>[5x]ALAGTIIAGASLTFQVLDKVLEELGKVSRKIAVGIDNESGGTWTALNAYFRSGTTDVILPEFVPNTKALLYSGRKDTGPVATGAVAAFAYY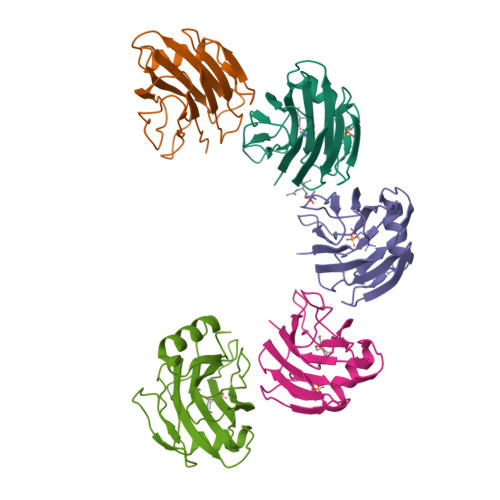MSSGNTLGVMFSVPFDYNWYSNWWDVKIYSGKRRADQGMYEDLYYGNPYRGDNGWHEKNLGYGLRMKGIMTSAGEAKMQIKISR>SLTCPQIKGNLTPCVLYLKNGGVLPPSCCKGVRAVNDASRTTSDRQSACNCLKDTAKGIAGLNPNLAAGLPGKCGVNIP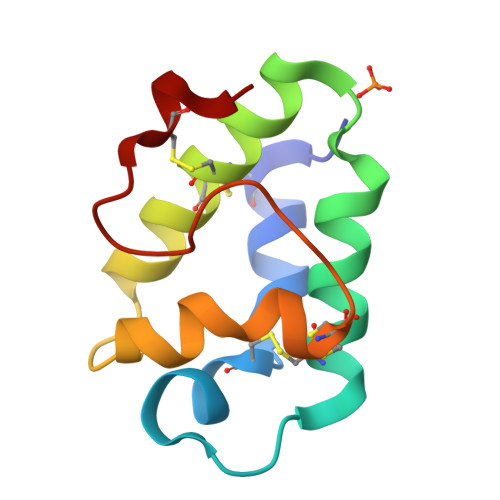YKISPSTNCNNVK[2x]>[2x]DYSLCQQREKLDDDMREMFTELHNGYRAAFARNYKTSKMRTMVYDCTLEEKAYKSAEKCSEEPSSEEENVDVFSAATLNIPLEAGNSWWSEIFELRGKVYNKNGKTSNIA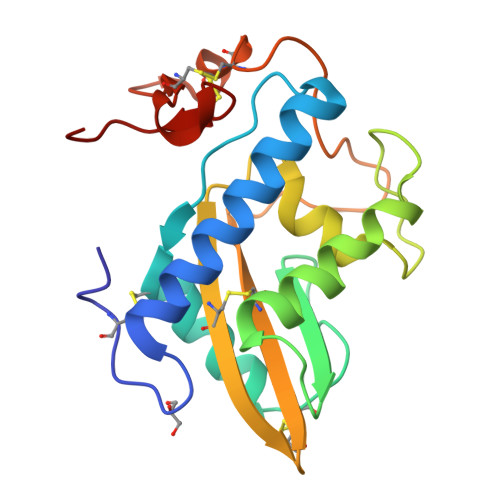NMVWDSHDKLGCAVVDCSGKTHVVCQYGPEAKGDGKTIYEEGAPCSRCSDYGAGVTCDDDWQNLLCIGHHHH(2S)-3-[(6-O-alpha-D-galactopyranosyl-beta-D-galactopyranosyl)oxy]-2-[(3Z,6Z,9Z,12Z,15Z)-octadeca-3,6,9,12,15-pentaenoyloxy]propyl 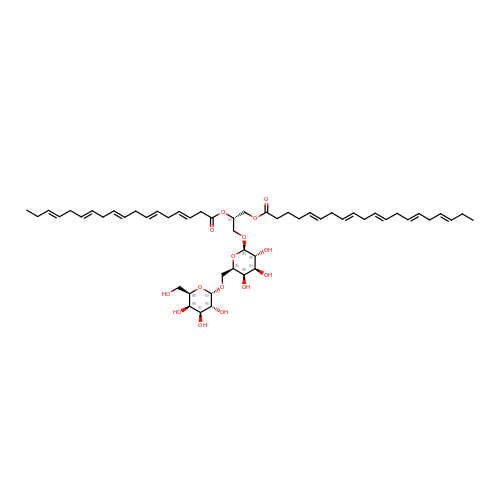(5Z,8Z,11Z,14Z,17Z)-icosa-5,8,11,14,17-pentaenoate | C53 H80 O15 | GBUVPODJTFTLEC-ZHVHOYJFSA-N> NSVTYNTLISGLGKAGRLEEALELFEEMKEKGIVPDVVTYNTLISGLGKAGRLEEALELFEEMKEKGIVPDVVTYTTLISGLGKAGRLEEALELFEEMKEKGIVPNVVTYTTLISGLGKAGRLEEALELFEEMKEKGIVPDVVTYTTLISGLGKAGRLEEALEL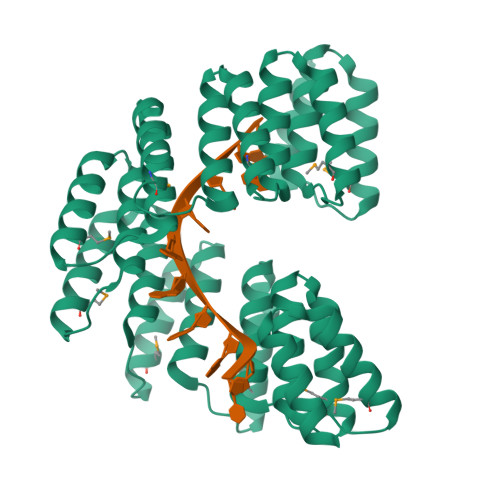FEEMKEKGIVPDVVTYTTLISGLGKAGRLEEALELFEEMKEKGIVPDVVTYNTLISGLGKAGRLEEALELFEEMKEKGIVPDVVTYNTLISGLGKAGRLEEALELFEEMKEKGIVPDVVTYTTLISGLGKAGRLEEALELFEEMKEKGIVPNVVTYTTLISGLGKAGRLEEALELFEEMKEKGIVPDVVTYTTLISGLGK>GQDMVSPPPPIADEPLTVNTGIYLIACYSLDDKAETFKVNAFLSLSWKDRRLAFDPVRSGVRVKTYEPEAIWIPEIRFVNVENARDADVVDISVSPDGTVQYLERFSARVLSPLDFRRYPFDSQTLHIYLIVRSVDTRNIVLAVDLEKVGKNDDVFLTGWDIESFTAVVKPANFALEDRLESKLDYQLRISRQYFSYIPNIILPMLFILFISWTAFWSTSYEANVTLVVSTLIAHIAFNILVETNLPKTPYMTYTGAIIFMIYLFYFVAVIEVTVQHYL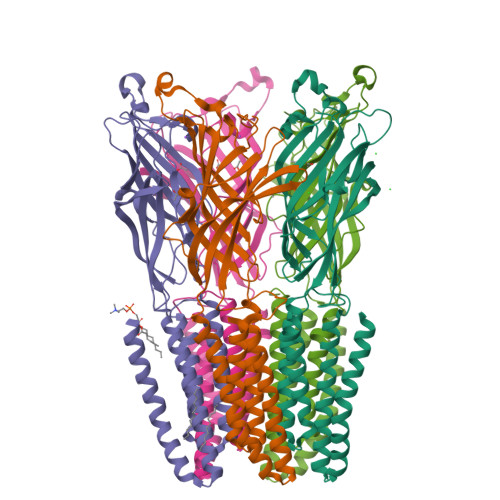KVESQPARAASITRASRIAFPVVFLLANIILAFLFFGF[5x]>[6x]MSNLPVEPEFEQAYKELASTLENSTLFQKNPEYRKALAVVSVPERVIQFRVVWENDKGEVQVNRGFRVQFNSALGPYKGGLRFHPSVNLSILKFLGFEQIFKNALTGLNMGGGKGGSDFDPKGKSDSEIRRFCVAFMTELCRHIGADTDVPAGDIGVTGREIGYLFGQYRKLRNSWEGVLTGKGGSWGGSLIRPEATGYGVVYYVEHMIAHATNGAESFAGKRVAISGSGNVAQ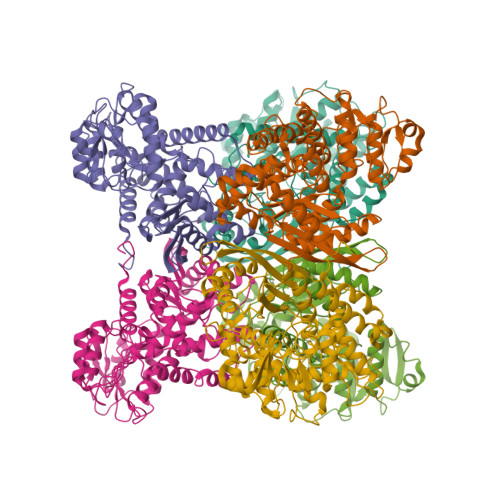YAALKVIELGGRVVSLSDSQGSLIVKDTAKDSFTPAEIDAIAALKVDRKQIAELVTDAAFADKFTYLPGQRPWVHVGAVDVALPSATQNEVSGEEAQALIAAGCKFIAEGSNMGCTQAAIDAFEAHREANKGAAAIWYAPGKAANAGGVAVSGLEMAQNSARLSWTAEEVDARLKDIMKSCFQNGLDTAKEYATPADGILPSLVTGSNIAGFTKVAAAMKDQGDWW> XYGIKKEIEAIKKEQEAIKKKIEAIEKELRQLANETTQALQLF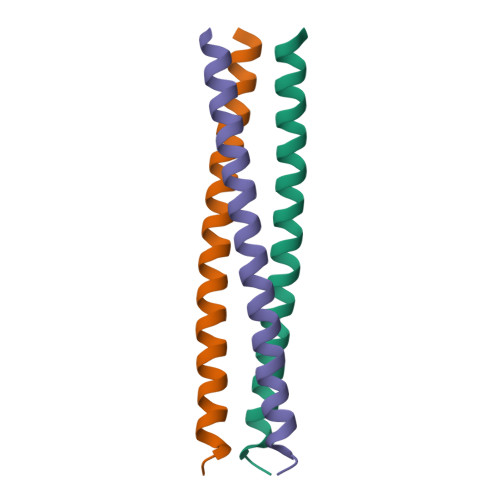LRATTEX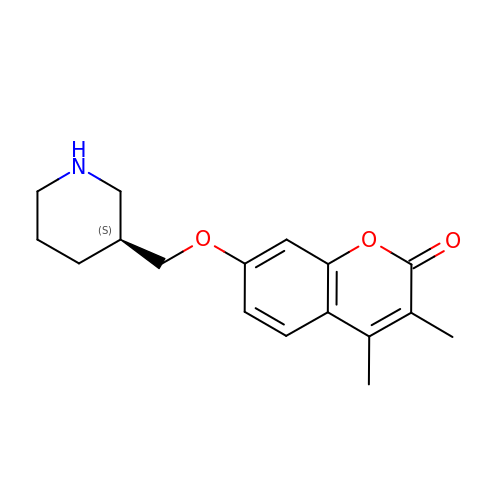3,4-dimethyl-7-[[(3~{S})-piperidin-3-yl]methoxy]chromen-2-one | C17 H21 N O3 | YHENGJCSDIHDOJ-ZDUSSCGKSA-N>[3x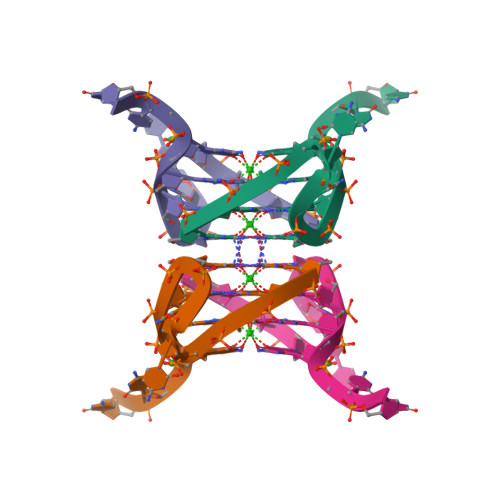]GGGGCCGGGGCC>MKFGEHLSKSLIRQYSYYYISYDDLKTELEDNLSKNNGQWTQELETDFLESLEIELDKVYTFCKVKHSEVFRRVKEVQEQVQHTVRLLDSNNPPTQLDFEILEEELSDIIADVHDLAKFSRLNYTGFQKIIKKHDKKTGFILKPVFQVRLDSKPFFKENYDELVVKISQLYDIARTSGAGSDGFTVLSTKSLFLGQKLQVVQADIASIDSDAVVHPTNTDFYIGGEVGNTLEKKGGKEFVEAVLELRKKNGPLEVAGAAVSAGHGLPAKFVIHCNSPVWGAD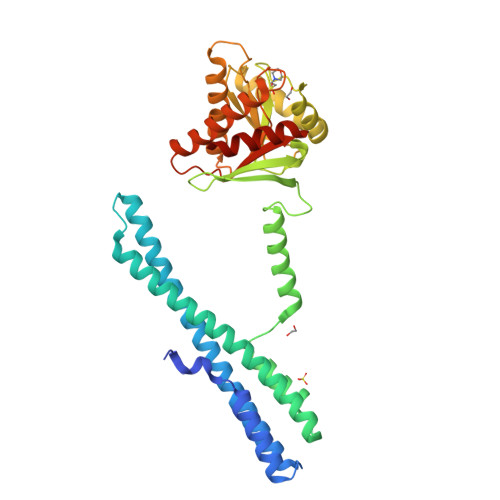KCEELLEKTVKNCLALADDKKLKSIAFPSIGSGRNGFPKQTAAQLILKAISSYFVSTMSSSIKTVYFVLFDSESIGIYVQEMAKLEHHHHHH[4x]>[2x]SNAGRYEIRFSGAGGQGLILAGVIMAEAASIYDGKQAVQSQSYGPEARGGASKSEVIISDGPVDYPKATQCDALLALTQEACDKYSADLKEGGVLLVDSDLVTKLPPGNYQTTAFNIIN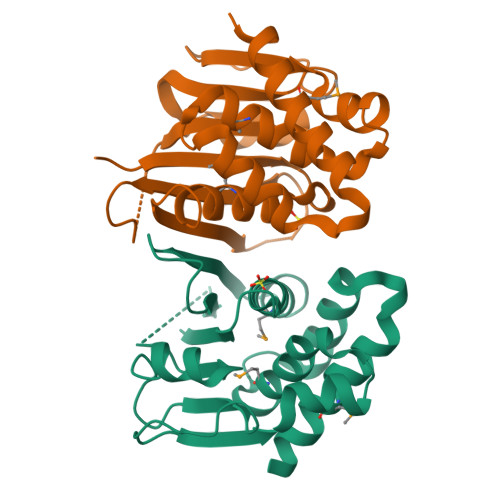TAKNDVGREIVANIVALGAMVALTGVVSKEAAEKAVLSRVPEAFVELNRKAFQMGFEKALAAKK> MNKFASFTTQYSLMLLIATLLSACGGSDGDDGSPGEPGKPPAMTISSLNISVDKVAISDGIAQVDYQVSNQENQAVVGIPSATFIAAQLLPQGATGAGNSSEWQHFTSETCAASCPGTFVDHKNGHYSYRFSATFNGMNGVTFLSDATQRLVIKIGGDALADGTVLPITNQHYDWQSSGNMLAYTRNLVSIDTCNSCHSNLAFHGGRYNQVETCVTCHNSKKVSNAADIFPQMIHSKHLTGFPQSISNCQTCHADNPDLADRQNWYRVPTMEACGACHTQINFPAGQGHPAQTDNSNCVACHNADWTANVHSNAAQTSALAQFNASISSASMDANGTITVA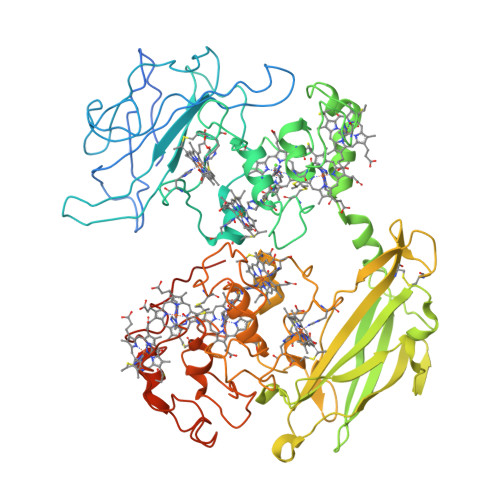VSLTNPTTGTAYADSADKLKFISDLRIYANWGTSFDYSSRSARSIRLPESTPIAGSNGTYSYNISGLTVPAGTESDRGGLAIQGRVCAKDSVLVDCSTELAEVLVIKSSHSYFNMSALTTTGRREVISNAKCASCHGDQQLNIHGARNDLAGQCQLCHNPNMLADATATNPSMTSFDFKQLIHGLHSSQFAGFEDLNYPGNIGNCAQCHINDSTGISTVALPLNAAVQPLALNNGTFTSPIAAVCSNCHSSDATQNHMRQQGAVFAGTKADATAGTETCAFCHGQGTVADVLKVHPINKGELKLEGKPIPNPLLGLDSTRTGHHHHHH> MDETDEDEFTPRPYQVELLERAMKKNTIVCLGTGSGKTFIAVMLIKELAHEIRGPFNEGGKRTFFLVNTVPLVNQQAKVIRKHTSLKVGEYVGDMGVDSWNKEKWNQEFEKHQVLVMTAQIFLDILNHGFISLSQVNLLIFDECHHAVKNHPYRQIMRHYKNLEQNDRPRILGLTASVINSKCKPNQVEKKIKELEATLNSR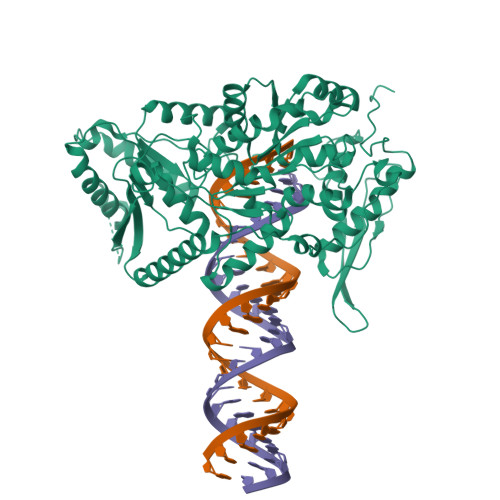VVTASDLEEVAVQKYATKPKEIIVSYNSDRKSDTSEVIENIINQALEQLSNIEETSNLNDTNSLKQIKKVLRDIKNILDELGPWCAHRVIKSRIRQLEKRESETAEELRTIRELLQSIFEQIINVLKNLEKLQKNNSVEFVSPKVKKLLEILKQYFSNNNNSSKELCGIIFVERRYTAYVLYKLLNELSAKRDDDFSFIKCDFVVGHNSSPSSKEKSTEMNSKKQKEVLKKFRKGECNLLVATSVVEEGIDIPKCNLVVRFDLPKNFRSYVQSKGRARAKNSKYIIMVEEDEKNKFQEDLNQYQEIEKILLRLCHNRDAPSEEDFDSFEDELLPPYMPYGTDGPRVTMSSAISLLHRYCSKLPSDRFTTLTPKFTYIEQNNEEENKMFRCTLRLPINSPLREPITGQPMPSKKLAKRSAALEACKKLHEMGELDDHLLPVKISRKNAELK> SDRAEVRNIPFKLGMSLTVGGVVNSNATRFSINVGESTDSIAMHMDHRFSYGADQNVLVLNSLVHNVGWQQEERSKKFPFTKGDHFQTTITFDTHT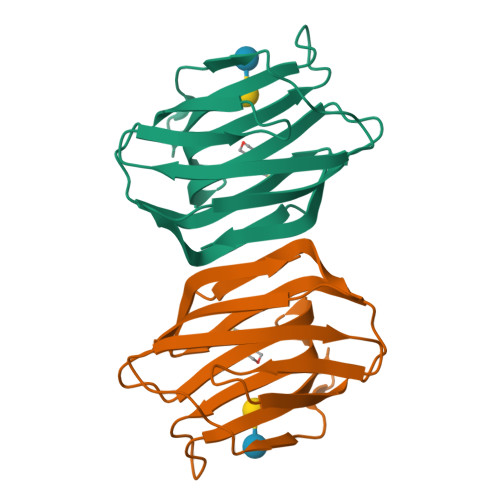FYIQLSNGETVEFPNRNKDAAFNLIYLAGDARLTFVRLE>[4x]MRNGLLKVAALAAASAVNGENLAYSPPFYPSPWANGQGDWAEAYQKAVQFVSQLTLAEKVNLTTGTGWEQDRCVGQVGSIPRLGFPGLCMQDSPLGVRDTDYNSAFPAGVNVAATWDRNLAYRRGVAMGEEHRGKGVDVQLGPVAGPLGRSPDAGRNWEGFAPDPVLTGNMMASTIQGIQDAGVIACAKHFILYEQEHFRQGAQDGYDISDSISANADDKTMHELYLWPFADAVRAGVGSVMCSYNQVNNSYACSNSYTMNKLLKSELGFQGFVMTDWGGHHSGVGSALAGLDMSMPGDIAFDSGTSFWGTNLTVAVLNGSIPEWRVDDMAVRIMSAYYKVGRDRYSVPINFDSWTLDTYGPEHYAVGQGQTKINEHVDVRGNHAEIIHEIGAASAVLLKNKGGLPLTGTERFVGVFGKDAGSNPWGVNGCSDRGCDNGTLAMGWGSGTANFPYLVTPEQAIQREVLSRNGTFTGITDNGALAEMAAAASQADTCLVFANADSGE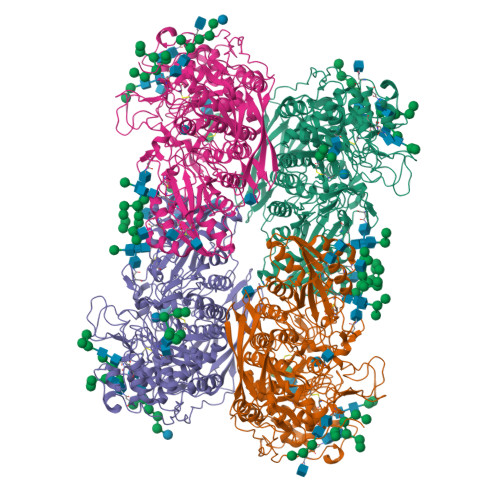GYITVDGNEGDRKNLTLWQGADQVIHNVSANCNNTVVVLHTVGPVLIDDWYDHPNVTAILWAGLPGQESGNSLVDVLYGRVNPGKTPFTWGRARDDYGAPLIVKPNNGKGAPQQDFTEGIFIDYRRFDKYNITPIYEFGFGLSYTTFEFSQLNVQPINAPPYTPASGFTKAAQSFGQPSNASDNLYPSDIERVPLYIYPWLNSTDLKASANDPDYGLPTEKYVPPNATNGDPQPIDPAGGAPGGNPSLYEPVARVTTIITNTGKVTGDEVPQLYVSLGGPDDAPKVLRGFDRITLAPGQQYLWTTTLTRRDISNWDPVTQNWVVTNYTKTIYVGNSSRNLPLQAPLKPYPGI> GSRVTEQDKAI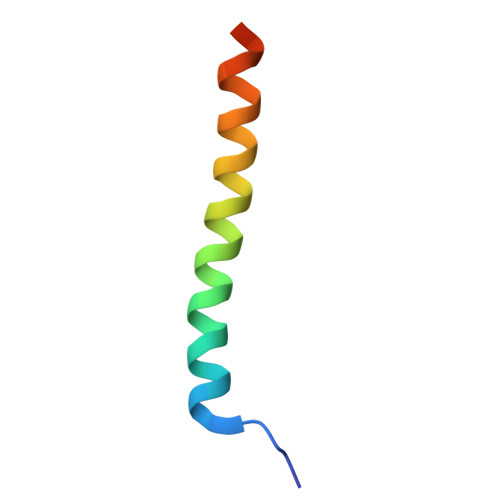LQLKQQRDKLRQYQKRIAQQLERERALA>[4x]MKGFAMLGINKLGWIEKERPVAGSYDAIVRPLAVSPCTSDIHTVFEGALGDRKNMILGHEAVGEVVEVGSEVKDFKPGDRVIVPCTTPDWRS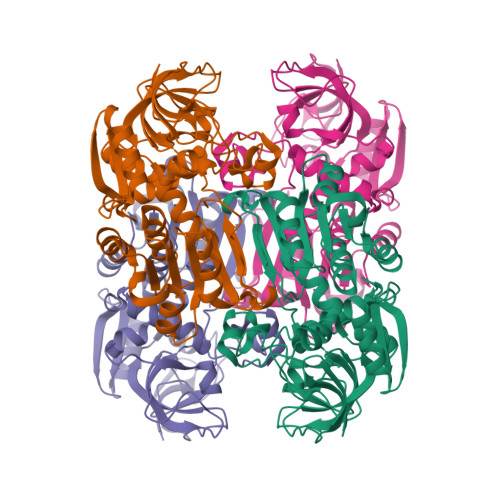LEVQAGFPQHSNGMLAGWKFSNFKDGVFGEYFHVNDADMNLAILPKDMPLENAVMITDMMTTGFHGAELADIQMGSSVVVIGIGAVGLMGIAGAKLRGAGRIIGVGSRPICVEAAKFYGATDILNYKNGHIVDQVMKLTNGKGVDRVIMAGGGSETLSQAVSMVKPGGIISNINYHGSGDALLIPRVEWGCGMAHKTIKGGLCPGGRLRAEMLRDMVVYNRVDLSKLVTHVYHGFDHIEEALLLMKDKPKDLIKAVVIL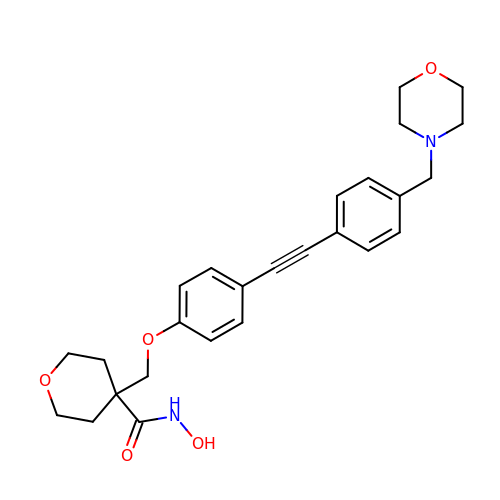N-hydroxy-4-[(4-{[4-(morpholin-4-ylmethyl)phenyl]ethynyl}phenoxy)methyl]tetrahydro-2H-pyran-4-carboxamide | C26 H30 N2 O5 | RGQLOHCHGMQBNF-UHFFFAOYSA-N>AGIKKMVAPSSAVEQCVVSVVHGNTQLNGLWLNDYVLCPRHILGKYTGEQWRDALINANNFDFHILYKGMELQVVGRELVGALLKLKVSMVNANTPKYKFAKARIGDNFSIACAYNGHVSGLYTVTLRENGTLKGSFMSGSCGSVGYNVTNEGVEFVYMHHLELPGCVHGGS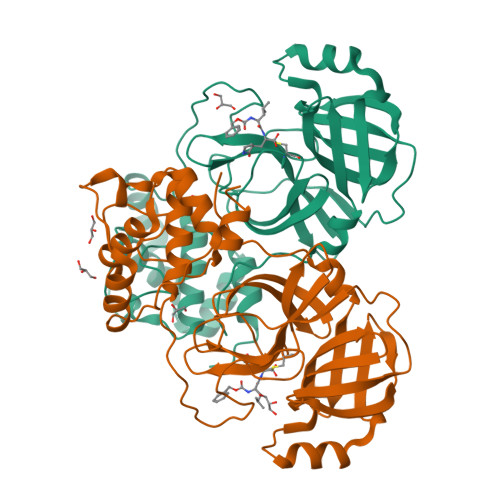DLHGIFYGGYVDEEVLQRIPPAPANSRNIVAWLYAAVYNNCDWFVKYGPKQVMSVEDFNEWASGYGFTKFEYHLAFDVFSAATGVSVEQMLAAIKELADGWNYAPVLGSFHLDDEYSPEMIMQQTSGIVLQ[2x]>[2x]GRGRRRRLVWTPSQSEALRACFERNPYPGIATRERLAQAIGIPEPRVQIWFQNERSRQLRQHRRESRPWPGRRGPPEGRRKRTAVTGSQTALLLRAFEKDRFPG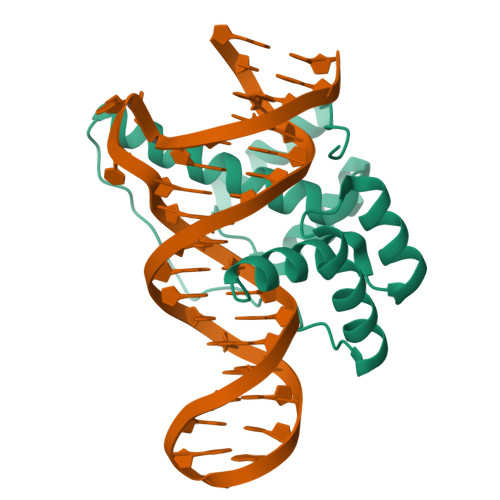IAAREELARETGLPESRIQIWFQNRRARHP>GSKPHQWQADEEAVRSATCSFSVKYLGCVEVFESRGMQVCEEALKVLRQSRRRPVRGLLHVSGDGLRVVDDETKGLIVDQTIEKVSFCAPDRNHERGFSYICRDGTTRRWMCHGFLACKDSGERLSHAVGCAFAVCLERKQ[2x];>[2x]QQKLPTNPFEVLR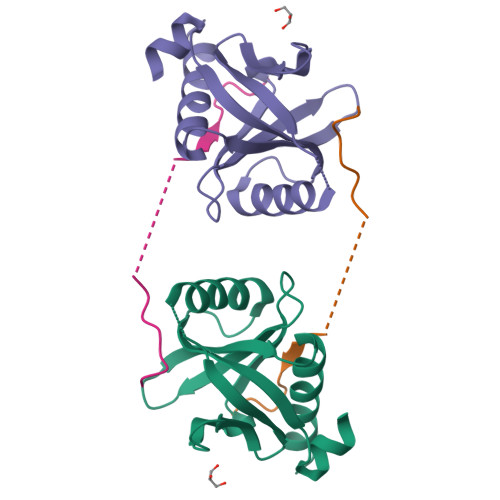QPPKKKKREHACFENPGLNLE The filamentous soft-rot fungus Hypocrea jecorina (previously Trichoderma reesei) secretes large quantities of carbohydrate degrading enzymes that act synergistically to degrade cellulose and related plant biomass components. One of these newly identified proteins that were found to be co-regulated with the major H. jecorina cellulases was a protein that was denoted Cellulose induced protein 1 (Cip1). The co-regulation of Cip1 with the other cellulase components in the fungus, and the fact that it contains a CBM, points towards a role (catalytic or carbohydrate binding) for Cip1 in the degradation of complex cellulose substrates. The Cip1 core domain structure is best classified as having a β-sandwich jelly-roll fold.

The two β-sheets consist of a total of 15 β-strands, eight in β-sheet A and seven in β-sheet B. One of these β-sheets (B) forms the floor of a large cleft and in the lower part of the molecule there is a “grip”-like motif where part of the other β-sheet (A) forms the “palm” and a protruding loop forms the “bent fingers”. A calcium atom was found to provide the best fit with regards to both B factor and metal coordination geometry. The calcium ion in the structure of Cip1 is hepta-coordinated and bound to seven oxygen ligands. The side chains of Glu7, Ser37 and Asp206 provide four of these, the latter bindjng in a bidentate mode with both oxygen atoms. The other three ligands consist of the carboxylic main chain oxygen atoms of Asp5, Ser37 and Asn40. Thus, it is clear that the removal of the calcium ion by addition of EDTA significantly affects the reversibility of the unfolding transition and this is consistent with a structural role for calcium in Cip1. Cip1 was treated with EndoH prior to crystallisation, trimming the glycosylation to leave only one bound N-acetyl glucosamine molecule. This can be seen in the structure, where Asn156 binds a NAG on the surface of Cip1 just outside the “grip” region. To summarise, Cip1 has two major regions with structural similarity to lyases; the potential active site cleft, which resembles that of an alginate lyase from the Chlorella virus, and the “grip” motif, which binds calcium and resembles that of a glucuronan lyase from H. jecorina.

> QISDDFESGWDQTKWPISAPDCNQGGTVSLDTTVAHSGSNSMKVVGGPNGYCGHIFFGTTQVPTGDVYVRAWIRLQTALGSNHVTFIIMPDTAQGGKHLRIGGQSQVLDYNRESDDATLPDLSPNGIASTVTLPTGAFQCFEYHLGTDGTIETWLNGSLIPGMTVGPGVDNPNDAGWTRASYIPEITGVNFGWEAYSGDVNTVWFDDISIASTRVGCG>MYILFREMKNNWYSLAALLSTIYSRHLDVEARPVKFEEIKKFPPEKTIVAYSFMSFDLDTVREEVKTLKERGYTLIAGGPHVTADPEGCLRMGFDHVFTGDGEENILKFLMGERKKIFDGLEHHHHHH[6x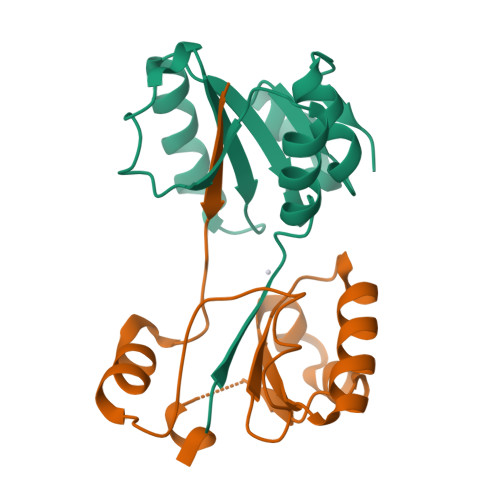]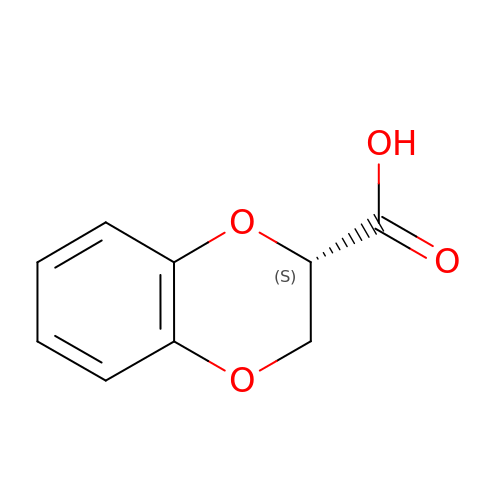(2S)-2,3-dihydro-1,4-benzodioxine-2-carboxylic acid | C9 H8 O4 | HMBHAQMOBKLWRX-QMMMGPOBSA-N> MYDWFSEMRKKDPVYYDGNIWQVFSYRYTKEVLNNFSKFSSDLTGYHERLEDLRNGKIRFDIPTRYTMLTSDP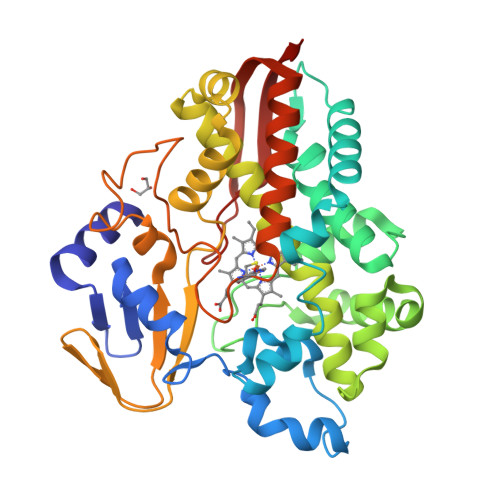PLHDELRSMSADIFSPQKLQTLETFIRETTRSLLDSIDPREDDIVKKLAVPLPIIVISKILGLPIEDKEKFKEWSDLVAFRLGKPGEIFELGKKYLELIGYVKDHLNSGTEVVSRVVNSNLSDIEKLGYIILLLIAGNETTTNLISNSVIDFTRFNLWQRIREENLYLKAIEEALRYSPPVMRTVRKTKERVKLGDQTIEEGEYVRVWIASANRDEEVFHDGEKFIPDRNPNPHLSFGSGIHLCLGAPLARLEARIAIEEFSKRFRHIEILDTEKVPNEVLNGYKRLVVRLKSNE>[3x]MNSQLTLRALERGDLRFIHNLNNNRNIM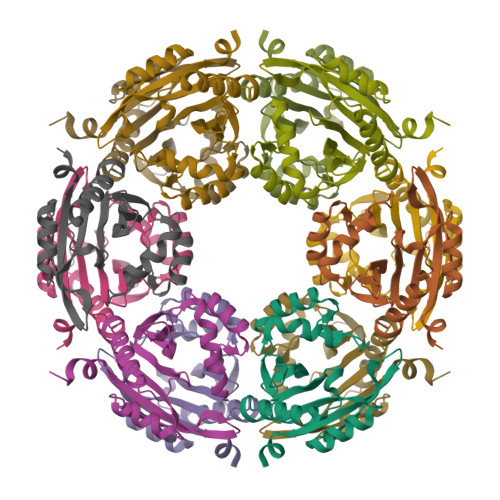SYWFEEPYESFDELEELYNKHIHDNAERRFVVEDAQKNLIGLVELIEINYIHRSAEFQIIIAPEHQGKGFARTLINRALDYSFTILNLHKIYLHVAVENPKAVHLYEECGFVEEGHLVEEAFINGRYQDVKRMYILQSKYLNRSE>[2x]MERAEILGVGTELLYGETLDTNTAEIARSLKPYALKVERTLRVADEVAPLAREVEEAFARARLVVLSGGLGPTPDDVTREAVALALGEPLELDEAVLGEIEAFFRAR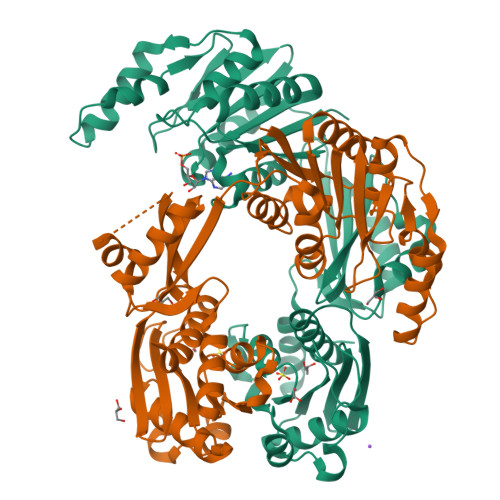GRAMPEANRKQAMRIPSATWLKNPRGTAPGWWVRKGGKDLVLLPGPPPEWRPMWQEVLPRLGLPRRPYAERVLKTWGIGESEIVERLGPLFVREEEVEVGTYPKVHGVEVVVRGREDRVAELAERIKKKLLKEVWGEGEMTLAEAVKRRMEREGATLSTMESLTGGLLGAEITRVPGASRFYLGGVVSYSVGAKARFGVPQDLLSRTVSAETARAMAEAARSLFGSTYALATTGVAGPDPLEGEPPGTVYVALAGPTGAEVRRYRFPGDRETVRLRSVYAALALLVT> GIEDLIDTAIKNALRVSQPPSTQSTEATSGVNSQEVPALTAVETGASGQAIPSDVVETRHVVNYKTRSESCLESFFGRAACVTILSLTNSSKSGEEKKHFNIWNITYTDTVQLRRKLEFFTYSRFDLEMTFVFTENYPSTASGEVRNQVYQIMYIPPGAPRPSSWDDYTWQSSSNPSIFYMYGNAPPRMSIPYVGIANAYSHFYDGFARVPL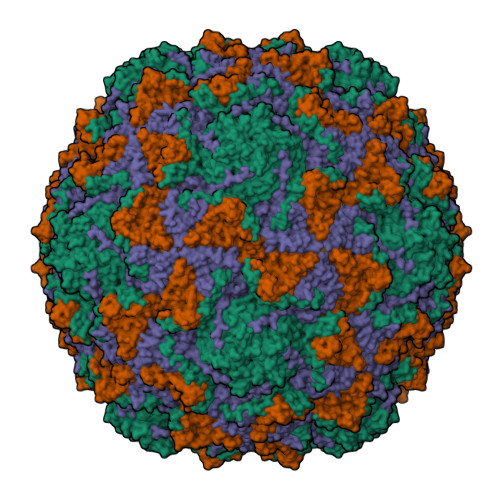EGENTDAGDTFYGLVSINDFGVLAVRAVNRSNPHTIHTSVRVYMKPKHIRCWCPRPPRAVLYRGEGVDMISSAILPLTKVDSITTF;> SPNVEACGYSDRVRQITLGNSTITTQEAANAIVAYGEWPTYINDSEANPVDAPTEPDVSSNRFYTLESVSWKTTSRGWWWKLPDCLKDMGMFGQNMYYHYLGRSGYTIHVQCNASKFHQGALGVFLIPEFVMACNTESKTSYVSYINANPGERGGEFTNTYNPSNTDASEGRKFAALDYLLGSGVLAGNAFVYPHQIINLRTNNSATIVVPYVNSLVIDCMAKHNNWGIVILPLAPLAFAATSSPQVPITVTIAPMCTEFNGLRNITVPVHQ;> GLPTMNTPGSNQFLTSDDFQSPCALPNFDVTPPIHIPGEVKNMMELAEIDTLIPMNAVDGKVNTMEMYQIPLNDNLSKAPIFCLSLSPASDKRLSHTMLGEILNYYTHWTGSIRFTFLFCGSMMATGKLLLSYSPPGAKPPTNRKDAMLGTHIIWDLGLQSSCSMVAPWISNTVYRRCARDDFTEGGFITCFYQTRIVVPASTPTSMFMLGFVSACPDFSVRLLKDTPHISQSKLIGRTQ;> GAQVSTQKTGAHENQNVAANGSTINYTTINYYKDSASNSATRQDLSQDPSKFTEPVKDLMLKTAPALN>EKREFDLSIEDTRIVLVGKRDFHTFAFNGQVPAPLIHVMEGDDVTVNVTNMTTLPHTIHWHGMLQRGTWQSDGVPHATQHAIEPGDTFTYKFKAEPAGTMWYHCHVNVNEHVTMRGMWGPLIVEPKNPLPIEKTVTKDYILMLSDWV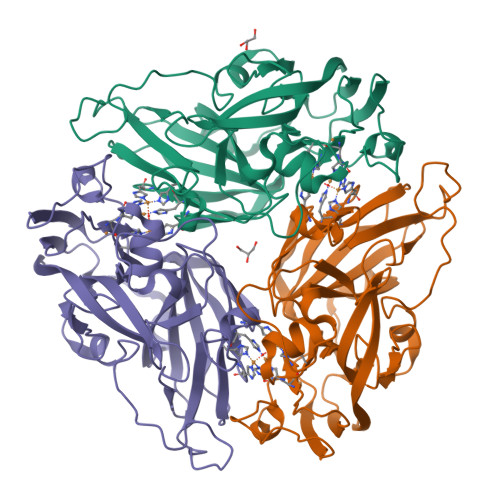SSWANKPGEGGIPGDVFDYYTINAKSFPETQPIRVKKGDVIRLRLIGAGDHVHAIHTHGHISQIAFKDGFPLDKPIKGDTVLIGPGERYDVILNMDNPGLWMIHDHVDTHTTNGDKPDGGIMTTIEYEEVGIDHPFYVWKDKKFVPDFYYEESLKKDLGMHNSKVFKGEPI[6x]> GGGIKMDTQFYDSFTFDNVKYSLYDNVYLFKS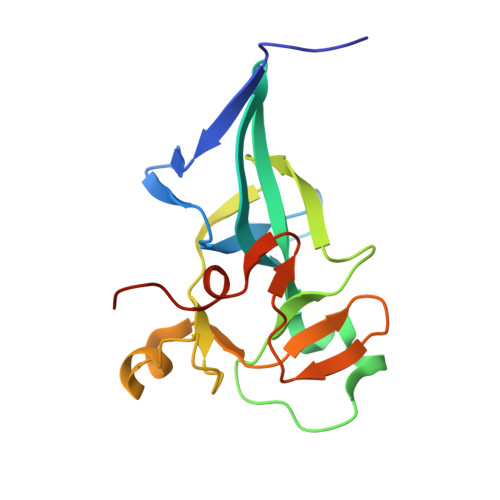GESEPYIGKIIKIWQQNQAKKVKILWFFLPDEIRKHLSGPVMEKEIFLACGEGVGLADINPLEAIGGKCTVLCISKDERNRQPSPRELAMADYIFYRFFDVNSCTLSEQLPEKIAGVEGNLLLNSKVEQVTSCS> 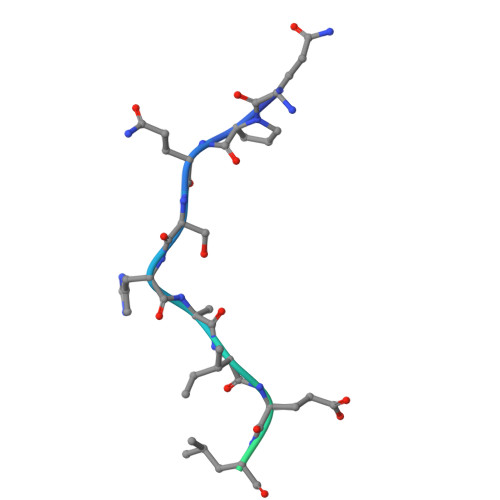QPQSHSIELDEVSKEAASTRAALTSNL> MSRNQDVFPILDLQELVICLQSCDFALATQENISRPTSDYMVTLYKQIIENFMGISVESLLNSSNQETGDGHLQEENENIYLDTLNVLVLNKICFKFFENIGVQDFNMTDLYKPEAQRTQRLLSAVVNYARFREERMFDCNSFILQMESLLGQLRSKFDDYNLIQQQLKQYEDVDGDNIPDEQELQKLEEQNKELEIQLKKLTKIQETLSIDYNDYKISKQSIFKDLEALSFQIVELESNRDKLIKISNTDMEELSEGIKELNDLLIQRKKT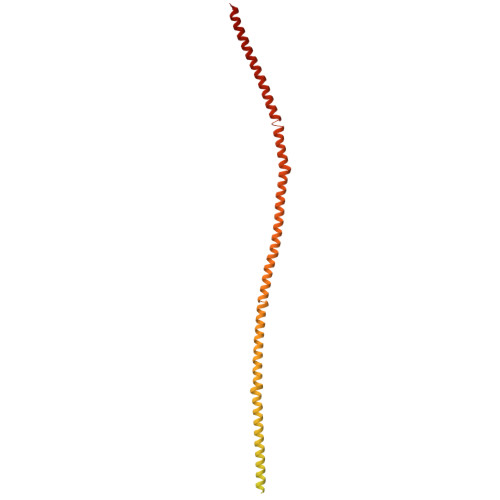LDDLTAQQKNLQDTVTTFETIISELYDVLRIISSEVQESNRTETELVGLKQNLINNKLKLMNVLETGIMYKLEILQEQLDLQLKNLEKLSQDTKEESRLNDTKLMDLQIKYENEIKPKIDKTDIFIQEELISGKINKLNDEIKQLQKDFEVEVKEIEIEYSLLSGHINKYMNEMLEYMQ> MASEDGEMPSQFEGIDPEQLTESQMQQYMMEMQRQGLLDSNMEGGQYEEGYEEGQEGEGYGEEYGDQDYDGNQNEYDSQQDSQQQGHDQVNEMHQDRYDRRVNSEISGNYEADDETLRKIRRDLLDNINLERRHRDLQPVYIDLTTNNISQYYSEYLVNNEHNQDFYENAKVRYNNLGECELCHITAKFEPDADITKEYIYDYFMEIGYLFLESEEEKRIILNPANNHIGIGVFFDEIQIVVVLILSEKVLCIQKISQPEQNKIEIRGKMLDENFGIYAIRIMNVDDQKKDIKGVGPEFIEYTRSTQEWMASFELELYNQDRMAIEYYTRVSPDSIPYKKKQSKNEKLTYKHLQLRLRTPFQIYPDPKYAAEDEKERIRKEQEILAHEEQERKEREENDAKRLKQSRKDYGDGQYDDDE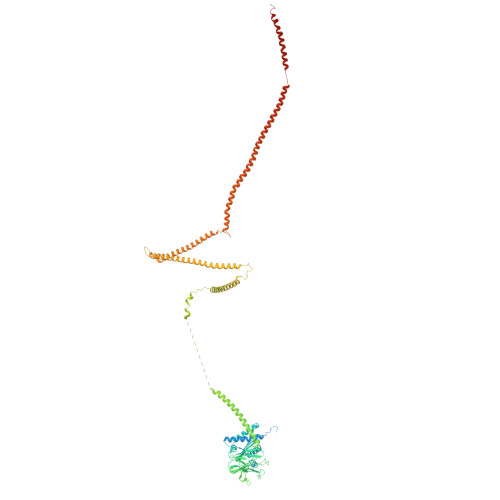HGQDDFNSQSDISDKDKHHDSMHAEQEQNQQAAQQQQDTISNKEIRQELEMAITEAQRQHDEFMLQNHKLQEEIKLLKNKNDGFVDRSNETAMNEHKYLNTLAHVHQIRLDLKQTQTRYNQMSQELQKKLEQKQKKCNEIKYAFLELKREVAKKAANSRTDKPIPEQQINEWEKAELQKSKELQELRLQILRLRNAYVKNQKILKKKEELAEGLHLIDFEQLKIENQTLNEKIEERNEELHKLKKKNTTTIQILTHTREKLGFVQGENGELNSQNVRKDQELDDMRKQLTQQKKTKDKLRSVNLTLKQQTGIVNSEELGQDYRDLRTRVSKLEEEKKRLEQKLRSMHEAIKTANQISTQNMQSQNNSLKKPYQPY> MVDGNYSVASNVMVPMRDGVRLAVDLYRPDADGPVPVLLVRNPYDKFDVFAWSTQSTNWLEFVRDGYAVVIQDTRGLFASEGEFVPHVDDEADAEDTLSWILEQAWCDGNVGMFGVSYLGVTQWQAAVSGVGGLKAIAPSMASADLYRAPWYGPGGALSVEALLGWSALIGTQLITSRSDARPEDAADFVQLAAILNDVAGAASVTPLAEQPLLGRLIPWVIDQVVDHPDNDESWQSISLFERLGGLATPALITAGWYDGFVGESLRTFVAVKDNADARLVVGPWSHSNLTGRNADRKFGIAATYPIQEATTMHKAFFDRHLRGETDALAGVPKVRLFVMGIDEWRDETDWPLPDTAYTPFYLGGSGAANTSTGGGTLSTSISGTESADTYLYDPADPVPSLGGTLLFHNGDNGPADQRPIHDRDDVLCYSTEVLTDPVEVTGTVSARLFVSS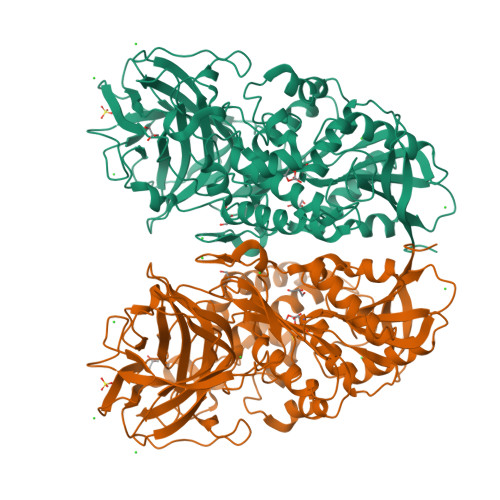SAVDTDFTAKLVDVFPDGRAIALCDGIVRMRYRETLVNPTLIEAGEIYEVAIDMLATSNVFLPGHRIMVQVSSSNFPKYDRNSNTGGVIAREQLEEMCTAVNRIHRGPEHPSHIVLPIIKRKLAAALEHHHHHH> GDLADRFAELERRYDARLGVYVPATGTTAAIEYRADERFAFCSTFKAPLVAAVLHQNPLTHLDKLITYTSDDIRSISPVAQQHVQTGMTIGQLCDAAIRYSDGTAANLLLADLGGPGGGTAAFTGYLRSLGDTVSRLDAEEPELNRDPPGDERNTTTPHAIALVLQQLVLGNALPPDKRALLTDWMARNTTGAKRIRAGFPADWKVIDKTGTGDYGRANDIAVVWSPTGVPYVVAVM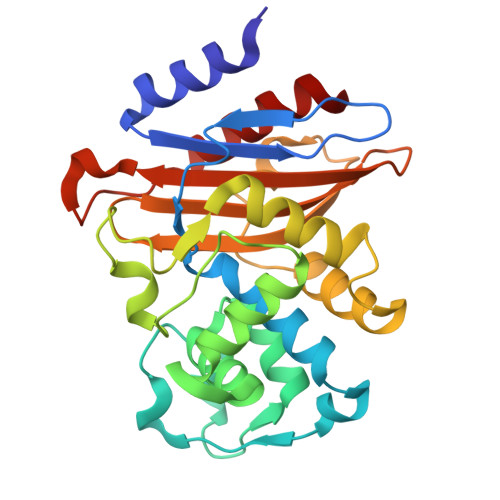SDRAGGGYDAEPREALLAEAATCVAGVLA> MEYSNPVIKGFYPDPSICRVGSDYYLVTSSFQYFPGVPIFHSTNLINWNKIGYCLIRPSQLMLNNATNRSGIFAPTLRYHEGIFYLITTNVTLKKNFIVMSEDLQGEWSEPIWIDGWGGIDPSLFFDNDGKVYITGTNDNARGEELGIYQAEIDLKKGSIIGERKLIWKGTGGSYPEAPHLYKVNGWYYLLIAEGGTEYGHMVTVARSKYPFGPFESCPFNPILTHRSTNHPLQAIGHADIVQYHDGSWWAVFHGTRPISYPPKHHLGRETCLAPIKWTDDGWPIIGYNGRIDIKMDAGYLPVKEKNIGDEIIEDDFNSDIFSTDWNFIQNPRLEHYSLKGRPSWLKMRGTEKTLNDINSPTFIGRRQEHFVCNVSTLLEFKPNQDNEEAGLTVYMNEKHHYEIALTKKNGRINVVLKKTVGDIQVVVNSLEYFSNTIIFSIQANPEEYKFSFVDPNTGQTYLLGTGLTTLLSTEVAGGFTGVYFGLYATGNGKVCTAPAFFDWFKYIPEIKGELNSKLEGKPIPNPLLGLDSTRTGHHHHHH

The β-1,4-xylosidase from the thermophilic bacterium Geobacillus thermoleovorans IT-08 (Xyl; GenPept accession No. ABC75004; EC 3.2.1.37) was found to be stable up to 55°C. The enzyme has a broad substrate specificity, and is active toward various xylans, xylooligosaccharides, as well as the artificial substrates p-nitrophenyl-β-D-xylopyranoside and p-nitrophenyl-α-L-arabinofuranoside in the pH range of 5.0–7.5. As observed in other type II GH43 enzymes, Xyl has two domains, an N-terminal five-bladed β-propeller catalytic domain (residues 1–304) and a C-terminal β-sandwich domain (residues 311–511). The active site of Xyl is located at the narrow end of the funnel-shaped central cavity of the five-bladed β-propeller domain. On the other hand, the residues in subsite -1 are fully conserved, including the catalytic base Asp-14, the catalytic acid Glu-177, and Asp-121, which modulates the pKa of the catalytic acid and keeps it in the correct, productive orientation.

X-ray diffraction data sets from Xyl, Xyl•arabinose, Xyl•xylose, and Xyl•arabinose•xylose crystals were collected to resolutions of 1.70, 2.10, 1.90, and 1.70 Å, respectively. Additional electron density in the Xyl structure suggested the presence of five independent glycerol molecules, of which two were in the active site. Of the five glycerol molecules in the Xyl structure, the one in subsite -1 exhibited the lowest average B-factor (10.4 Å2). In the Xyl structure, 7 amino acid side chains (Ser-4, Ser-22, Asn-49, Met-100, Asp-293, Val-426, and Ser-441) were modeled in two alternate conformations. In total 570, 471, 531, and 516 water molecules were identified and refined in the final models of Xyl, Xyl•arabinose, Xyl•xylose, and Xyl•arabinose•xylose, respectively. One calcium ion was defined in each final model on the basis of its electron density, coordination geometry (pentagonal bipyramid) and positional similarity to other GH43 protein structures. A metal ion is bound to the carbonyl oxygen atoms of Asp-316 and Asp-503, and the Ser-344 Oγ and Asp-503 Oδ1 atoms, with three water molecules complementing the coordination sphere. The calcium ion likely has a stabilizing function. In contrast to all structurally characterized type II GH43 β-1,4-xylosidases, protein assembly analysis using the PDBePISA server suggested that Xyl from both crystal forms is probably stable in solution as a dimer.4-[(3R)-8,8-dimethyl-3,4-dihydro-2H,8H-pyrano[2,3-f]chromen-3-yl]benzene-1,3-diol 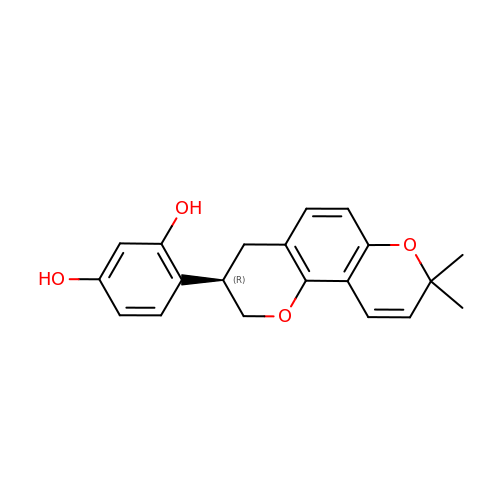| C20 H20 O4 | LBQIJVLKGVZRIW-ZDUSSCGKSA-N> MRKICIFLLVLFCGNVLRSQVKPAVQDTTKTQFSVGKMELENPPSILSAYKYDPITDRYIYTTSVDGFSIDYPLVLTPKEYEDLLLKESRRDYFRKKMDAIDGKKTGAEAAKKDLLPRYYINSSLFESIFGSNTIDVKPTGSVEMDLGVRYTKQDNPAFSPRNRSSLTFDFDQRISMSLMGKIGTRLEVNANYDTQSTFAFQNLFKLAYTPSEDDIIQKVEVGNVSMPLNSTLIRGAQSLFGVKTQLQFGRTTITGVFSEQKS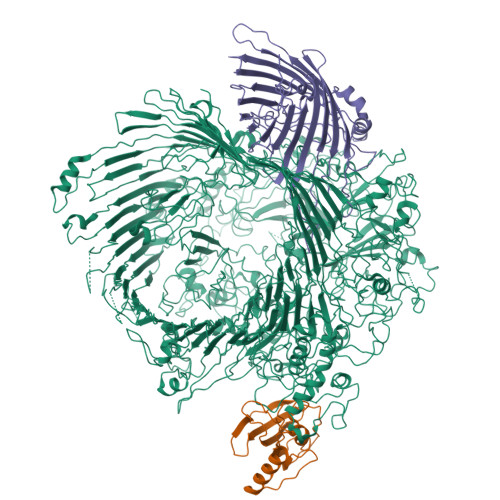QTKSVVAENGGTVQNFDLYALDYDNDRHFFLSQYFRNKYDVSLKNYPFIDSRVQITRLEVWVTNKQNRVTTTGGGNNLRNIIALQDLGEAQVSGVPDNEVVVISSTAGFFNNPIDSPTSNTNNKYDPATIGQAGSFLNSNIREIVTAKSGFNNTNVSEATDYSVLENARKLTTNEYTFNPQLGYISLQQRLANDEILAVAFEYTVGGKVYQVGEFGSDGVDATVVTGNNSSNQAIITQSLVLKMLKSNLTNVKNPVWNLMMKNVYQIPQAYQIKQDDFRLNILYTDPSPINYITPVQGSSFPPNPAPDSKVEQTPLLNVFNLDRLNYNNDPQAGGDGFFDYIPGVTVDVQNGRVIFTTKEPFGELIFNKLQTGAGESYNDPTTYNANQQKYVFRNMYRNTQAGALQDSDKNKFLLRGKYKSSGSNGIPIGAFNVPQGSVVVTAAGRVLVEGIDYSVDYQLGRVQILDPSLQASNTPIEVSLENNSIFGQQTRRFMGFNIEHKISDKFVIGGTYLKMTERPFTQKSTYGQESVNNTIFGFNGNYSTEVPFLTRLANKLPNIDTDVPSNLSIRGEVAFLRPDAPKASDFQGEATIYVDDFEGSQSTIDMRSAYAWSLASTPFITSINDNTFNANSNTLEYGFKRAKLSWYTIDPVFYSSKPSGISNDDLSLNTTRRIYSRELYPNTDIAQGQIQVVNTLDLTYYPGERGPYNNNPSFGASNPSANFGGIMRALNSTNFEQGNVEYIQFWVLDPYVGNGESPATNAGKIYFNLGEISEDVLKDGRKQYENGLGPDQVMVNPQPLWGDVPASQSLIYAFDTNPDNRKNQDVGLDGLPSSREGSIYTNYAGEADPAGDDYTYYLNADGGVLERYKNYNGTEGNSAVSINDPNRGSTTLPDVEDINRDNTMSTINAYYEYSIDVKPGMQVGENYITDIREVTNVDLPNGGTTNARWIQFKIPVSQPQNTIGNITDFRSIRFMRMFMTGFNSQMTVRFGALDLVRGEWRRYTGTLDANDQNPDDDGVEFDVAAVNIQENGTKCPVNYVMPPGVQREQLYNNNTVINQNEQALAVRIGGAGLQYQDSRAVFKNVSVDMRQYKKLKMFLHAESLPNQPTLEDDEMVGFIRFGNDFTQNFYQVEIPLKVTKTGGSCSISPDLVWMDDNSIDLALDLLTRMKIKAMSIDINSSKRDVNGIYYPDNDPDLEGGDGDGKLTLGIKGNPNFGLVRNLMVGVKSRADHKDIKGEVWFNELRLADLENKGGMAAILNVDTNMADFATVSATGRKSTIGFGSLEQGANERDREDVQQYNIVTNLNLGKLLPKKWGINLPFNYAIGEEVITPEYDPFNQDIKLDQLIRETTDQAEKDNIRTRAIDYTKRKSINFIGVRKDRAPEQKPHVYDIENFTFSQSYNQVERHDYEVADYEDEQSNSAVNYAYTFQPKEVVPFKSTKFMKKSEYWKLLSDFNFNYLPSNISFNTNILRQSNRQQFREVEVEGIGLDPLYRRNFAFNYQYGFGFNLTKSLKLNYSATSNNIVRNFLNDDNSPKEDFNIWDDYLDIGTPNQHAQQLVLNYDIPINKIPIFGFVKASYSYTADYMWQRSSTAFSEYEDPNGTVYDLGNTIQNSNSNTLTTTLNMNTLYKYLGLTPGAKKTAKPKTAAPPKPGEKIVNTAKPVVSSSPFYDGLIGVLTSIKNVQINYTKNSGTVLPGYTPSVGFLGTSKPSLGFVFGSQDDVRYEAAKRGWLTTYQDFNQSFTQVSNKLLKVTANIDLLPDLKVDLSMDRSYSENTSEQYSVDPSTNEYKPLSPYTYGMFSISTVMIKTAFSPSDETQSAAFDDFRSNRLIIANRLAEGHYGSGVAIPRYGDANNPIPAETDPNYAVYTANQGYPIGYTKSNQAVLLPAFLAAYTGSDASSSSTNIFRSFPIPNWSIKYNGLMRYKYFKDKFKRFSLQHNYRASYTINQFRSNFDYNSSPKVQDVNTNFYNEIIMSNVNLVEQFSPLIRMDFELKSSLRVLSEIKKDRALSMSFDNNLLTEVKGMEYIIGLGYRFKDVIFSSRLADNPTGIIKSDINIKADFSLRNNETLVRYLDYDNNQLAAGQNIWSLKLTADYSFSKNLTAIFYYDHSFSKAVISTSFPLTNIRSGFTLRYNFGN;> MKQLLTALLSLTLFISCSKDKDEVKDYTAENEKEIVDYLAQNNLTAQRTNSGLYYIITKEGSSESEGENPGEEENTGEGENTEENENDGHPTLNSNITVIYKGYFTNGKVFDESTEGVSYSLRTLIPGWKEGIPLLKSGGEIQLFVPAHLGYGSNGNKTVPGGAVLIFEITLVSVN;> MKKISLLLICLLITTFAKAQDIERPITTGVPFLLVAADARAAGLGDQGVATSSDVFSQQWNPAKYAFAEDAQGLSISYTPYLTDLANDISLGQVTYYNKINDRSAFAGSFRYFGFGGIELRQTGDPNEPTREVNPNEFALDGSYSLKLSETFSMAVAARYIRSNLKVATEEIDASAAGSFAVDVAGFYQSEEIAYSDFNGRWRAGFNIQNLGPKISYDHDDLSANFLPANLRVGGGFDFIFDDYNKLGVSLELTKLLVPTPPGPGTPYDANGDGDFTDPGDISQSQADEANYKKYKDIGWVSGIFKSFGDAPGGFSEELKEITYSAAAEYMYQDAFAMRLGYYHESPMKGAKQFFSLGAGFKYSMIKVDVSYLFSASKVKNPLENTLRFSLTFNFGDKYETY>[2x]MSTTDQGET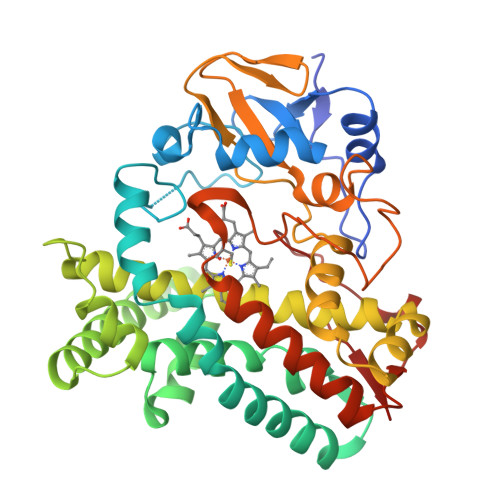GKACPYPFAEMERLEIHPEYNRLRDAGELGRVLMPYGGETWLATSWEDVAKVFVDPRFSRSATLGKDVPRVLPAIQDQPVIMLMDPPEHTRLRRLATKALTSRRMEALRPRTQEVADDLIDKMLAKGAPADLMEDFALPLPIIMICELLGVPIEDQTKFRTWSDQMLSNGAYSQEVVMAAGQSLYLYLSELIAERRKQDTNDLLGSLVRARDKDDRLSETELVGFAVTLLIAGYETTANAIGNSVYTLLTHPEKLAELRKDLSLIPKAVDELLRIIPIAKQASWVRMAVEDVELSGTIVKAGEAVAIQTHSANTDPKVYDHPEEIDFHRTSNPHMSLGHGAHHCMGAQLVRVEMQTALGSLISRIPALRFAVPEPRIKFLRGRLVPSLEALPLTW> MEKTRPDYTSFNTVDEWLEAIK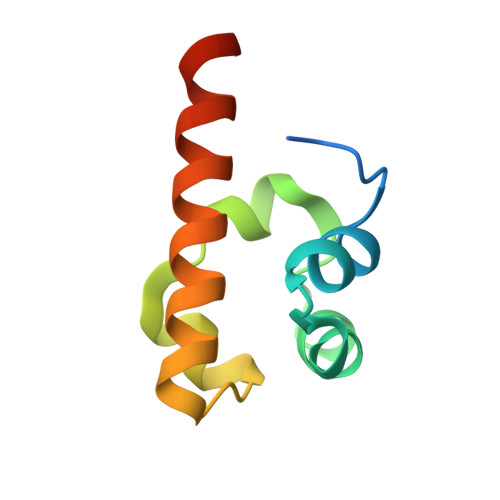MGQYKESFANAGFTSFDVVSQMMMEDILRVGVTLAGHQKKILNSIQVMRAQMNQIQSVEV>[2x]MHAGEAVQQLKKAFETVASFDFRDALSKASTPVTVVATNGPFGLAGLTCSAVCSVCDRPPTVLLCINRKSYAAGIIKSN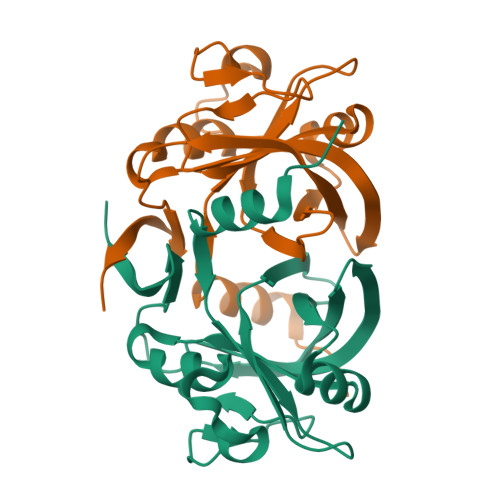GVLSVNWLAAGQAVISQTFAGVGSVPMEERFADKGWQTIATGAPYRMDAAVSFDCTIANIVDVGSHSVIFAEVVARNHAEECTPLIYHRRQYATTRSLAEHHHHHH> MAATSSSDSDGGKGESEANSKWLDSLSDSMANIHTFSACLALADFHGDGEYKLAMGDLGPDGRQPRLKVLKGHTLVSQKPLPDLPAAAVTFLMASHEPRTPALAIASGPCVYVYKNLKPYFKFSLPSLPTNPLEQDLWNQAKEDQIDPLTLKEMLEGIREKAEVPLSVQSLRFLPLELSEMEAFVNQHKSKSIRRQTVITTMTTLKKNLADEDAVSCLVLGTENKELLVLDPEAFTILAKMSLPSVPAFLEASGQFDVEFRLAAACRNGSIYILRRDSKRPKYCIELG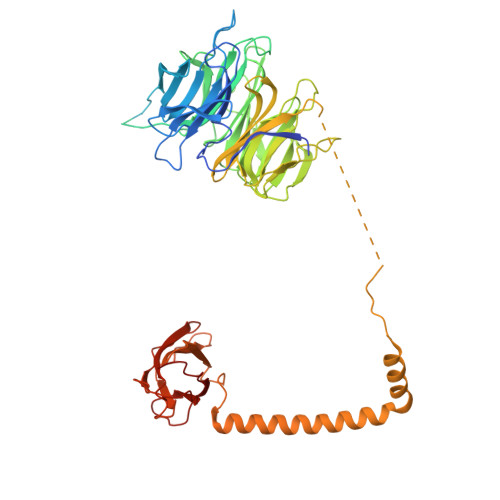AQPVGLVGVHKVLVVGSNQDSLHGFTYKGKRLWTVQMPAAILAMNLLEQHSRGLQAVMAALANEEVRIYHDKVLLNVIRTPEAVTSLCFGRYGREDNTLIMTTLGGGLIIKILKRTAVFAEGGGEAGPPPSQAIKLNVPRKTRLYVDQTLREREAGTAMHRTFQADLYLLRLRAARAYVQALESSLSPVSLTAREPLKLHAVVQGLGPTFKLTLHLQNTSTARPILGLVVCFLYNEVLYALPRAFFKVPLLVPGLNYPLETFVKSLSDKGISDIIKVLVLREGQSTPLLSAHINMPMSEGLAAD>MKALTARQQEVFDLIRDHISQTGMPPTRAEIAQRLGFRSPNAAEEHLKALARKGVIEIVSGASRGIRLLQEEEEGLPLVGRVAAGEPLLAQQHIEGHYQVDPSLFKPNADFLLRVSGMSMKDIGIMDGDLLAVHKTQDVRNGQVVVARIDDEVTVARLKKQGNKVELLPEN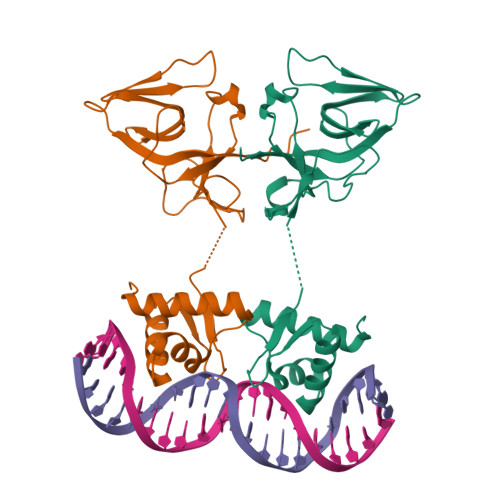SEFKPIVVDLRQQSFTIEGLAVGVIRNGDWL[2x]> TAHRFLFVSTPVGPLGSGRGGGVELTLPNLAKALTQRGHQVSVLAPAGSVLPDLPLETVPGTWQSTAQSHGRATPAEIPAESVLARLWDRAHQQQADFDLILNFAYDWLPLYLTPFFKTPVAHLISMGSLSEVMDQAIATSLDRYPGSIAVHSLAQAATFPFGDRCLCIGNALDLAAYGFNPEPEPVLGWVGRIAPEKGLEDAIQAAQQAGLPLRVWGALTEPDYWQRLQQQFGDRAVS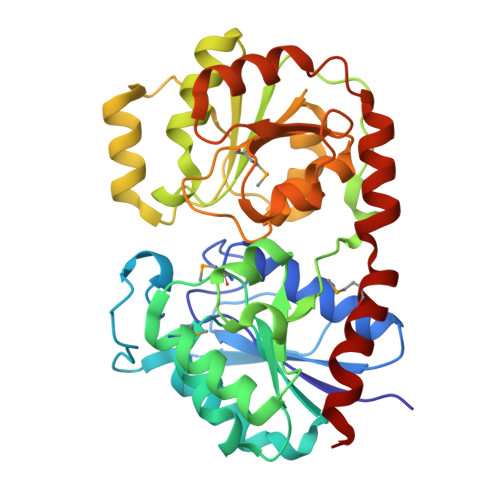YQGFVSTDELQRGLGRCQGLLMTPKWVEAFGNVAIEALACGLPVIAYARGGPLEIIEQGKSGWLVEPDQQAALVNAIGQLSSLDRAYCRAQAEARFSLAAMGQRLEAWLLPLLSR>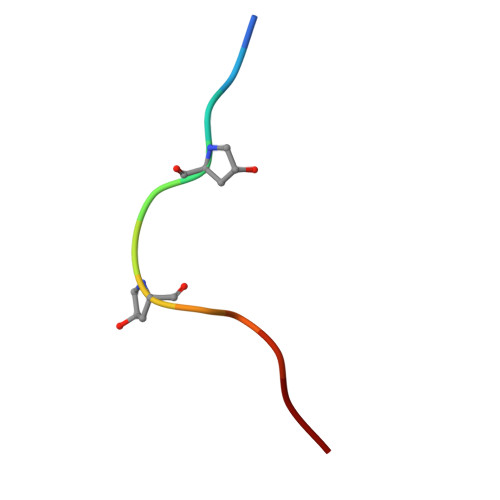 HEVPSGPNPISN> AGYPPASPSNLSCLMHLTTNSLVCQWEPGPETHLPTSFILKSFRSRADCQYQGDTIPDCVAKKRQNNCSIPRKNLLLYQYMAIWVQAENMLGSSESPKLCLDPMDVVKLEPPMLQALDIGPDVVSHQPGCLWLSWKPWKPSEYMEQECELRYQPQLKGANWTLVFHLPSSKDQFELC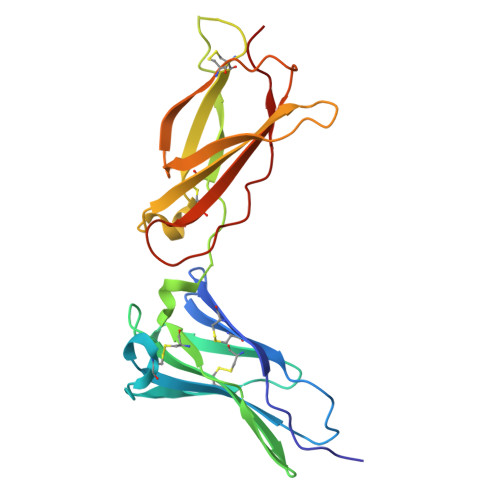GLHQAPVYTLQMRCIRSSLPGFWSPWSPGLQLRPTMKA>MTMPYYASAEQIMRDRSELARKGIARGRSVVVLTFRDGVLFVAENPSTALH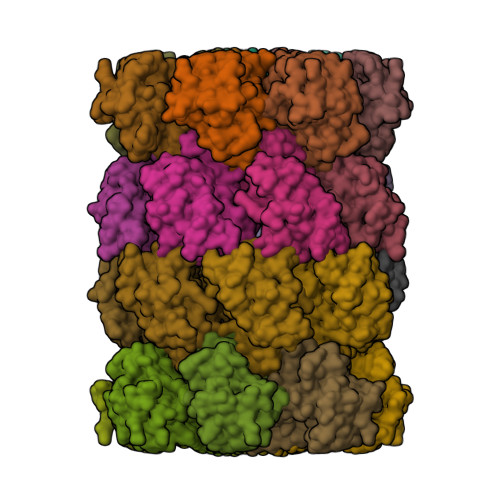KVSELYDRLGFAAVGKYNEFENLRRAGIVHADMRGYSYDRRDVTGRSLANAYAQTLGTIFTEQPKPYEVEICVAEVGRVGSPKAPQLYRITYDGSIVDEQHFVVMGGTTEPIATAMRESYRADLDLEAAVGIAVNALRQGGAGEGEKRNVDVASLEVAVLDQSRPRRAFRRIAGTALEQLVPAEPAAASESAPEPKPDTETKPADTQD[7x];>MTADRPALRTGDRDTRLSFGSNLSSFTDYLRGHAPELLPENRIGHRSHSTRGGDGMESGDLAPHGTTIVALTYKGGVLLAGDRRATQGNLIASRDVEKVYVTDEYSAAGIAGTAGIAIELVRLFAVELEHYEKIEGVPLTFDGKANRLASMVRGNLGAAMQGLAVVPLLVGYDLDADDESRAGRIVSYDVVGGRYEERAGYHAVGSGSLAAKSALKKIYSPDSDEETALRAAIESLYDAADDDSATGGPDLTRGIYPTAVTITQAGAVHVSEETTSELARRIVAERTEQGGSAR[7x]(1S,4R,9S)-5-(trifluoromethyl)-1,2,3,4-tetrahydro-1,4-methanonaphthalen-9-amine | C12 H12 F3 N 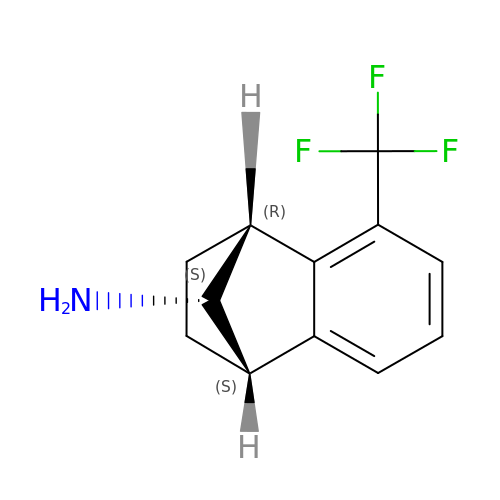| HHIJEPNAHYLKPE-RNSXUZJQSA-N> TPEAPYASLTEIEHLVQSVSKSY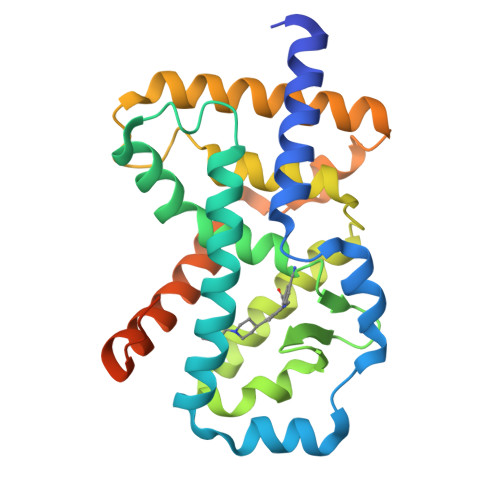RETCQLRLEDLLRQRSNIFSREEVTGYQRKSMWEMWERCAHHLTEAIQYVVEFAKRLSGFMELSQNDQIVLLKAGAMEVVLVRMCRAYNADNRTVFFEGKYGGMELFRALGCSELISSIFDFSHSLSALHFSEDEIALYTALVLINAHRPGLQEKRKVEQLQYNLELAFHHHLCKTHRQSILAKLPPKGKLRSLCSQHVERLQIFQHLHPIVVQAAFPPLYKELFSTETESPVGLS> NTRTIYLAGGCFWGLEAYFQRIDGVVDAVSGYANGNTKNPSYEDVSYRHTGHAETVKVTYDADKLSLDDILQYFFRVVDPTSLNKQGNDTGTQYRSG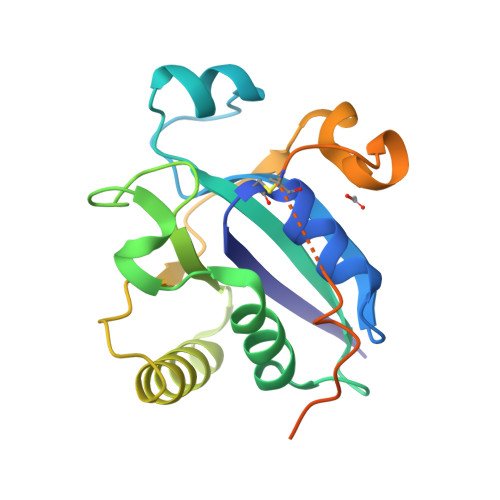VYYTDPAEKAVIAAALKREQQKYQLPLVVENEPLKNFYDAEEYHQDYLIKNPNGYCHIDIRKADEPLPGKTKTAPQGKGFDAATYKKPSDAELKRT>MHHHHHHHHHHLEVLFQGPSEFPMAQSNIIAGMDLNRLDRIAEHLDRAYLHPGKLAGTMTLVARRGEVVYCQAQGLRDVERQLPVERDTLFRIYSMTKPITSIALMQLYEQGRFLLDEPVHKYIPTWKNLRVYKTGSHPQMLTTAPQRPMTIRDLLTHQSGLTYGFMNRTNVDAAYRSLKLDGGPGHTLDRLIDELARLPLEFSPGTAWNYSVATDVCGYLVQLLSGMSLDDYFSKHIFQPLGMPDTFFTVPAEKLSRFAACYEYQPGDSFSLQDDPQGSAFAKAHGYLSGGGGLVSCVDDYYRFAQALANGGELDGARIIGRKTLEFMRMNHLPDNKGLPDVAIGSFSETPYDGTGFGLGFSVKLDVAKSQTVGSVGEYGWGGMASTNFFIDPEEDLLMVFMT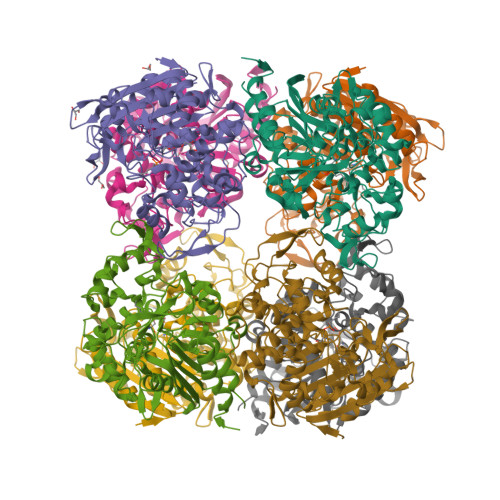QLIPSSTYAVRQELRAIINGALVDA[8x]> UCCCAGUCCACCGCGGUGAGAAGGG;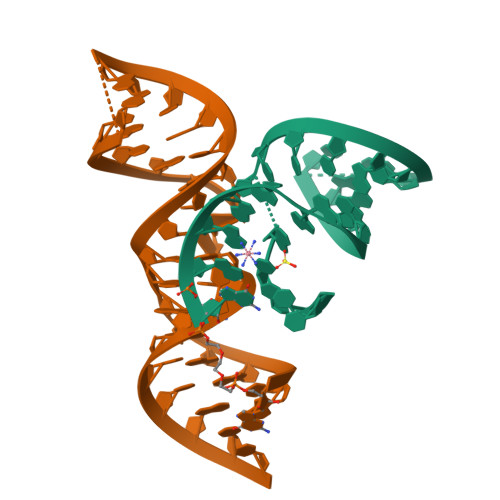> GGCAGAGAAACACACGAUCGUGGUACAUUACCUGCC>GGCACU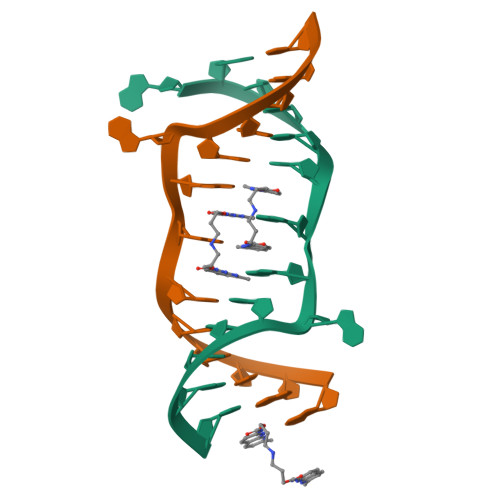GGAAGUGC[2x]>MAVKVEYDLKRLRNIGIAAHIDAGKTTTTERILYYTGRIHKIGEVHEGAATMDFMEQERERGITITAAVTTCFWKDHRINIIDTPGHVDFTIEVERSMRVLDGAIVVFDSSQGVEPQSETVWRQAEKYKVPRIAFANKMDKTGADLWLVIRTMQERLGARPVVMQLPIGREDTFSGIIDVLRMKAYTYGNDLGTDIREIPIPEEYLDQAREYHEKLVEVAADFDENIMLKYLEGEEPTEEELVAAIRKGTIDLKITPVFLGSALKNKGVQLLLDAVVDYLPSPLDIPPIKGTTPEGE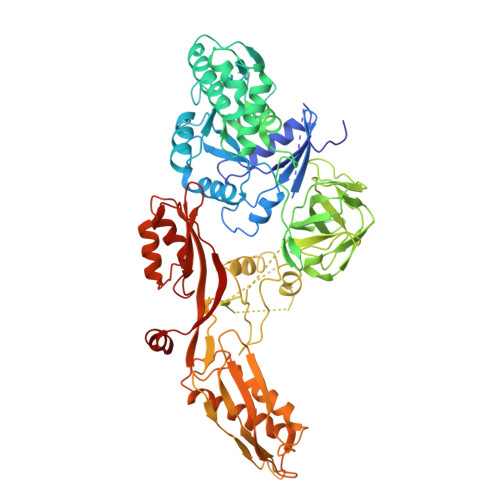VVEIHPDPNGPLAALAFKIMADPYVGRLTFIRVYSGTLTSGSYVYNTTKGRKERVARLLRMHANHREEVEELKAGDLGAVVGLKETITGDTLVGEDAPRVILESIEVPEPVIDVAIEPKTKADQEKLSQALARLAEEDPTFRVSTHPETGQTIISGMGELHLEIIVDRLKREFKVDANVGKPQVAYRETITKPVDVEGKFIRQTGGRGQYGHVKIKVEPLPRGSGFEFVNAIVGGVIPKEYIPAVQKGIEEAMQSGPLIGFPVVDIKVTLYDGSYHEVDSSEMAFKIAGSMAIKEAVQKGDPVILEPIMRVEVTTPEEYMGDVIGDLNARRGQILGMEPRGNAQVIRAFVPLAEMFGYATDLRSKTQGRGSFVMFFDHYQEVPKQVQEKLIKGQ[2x]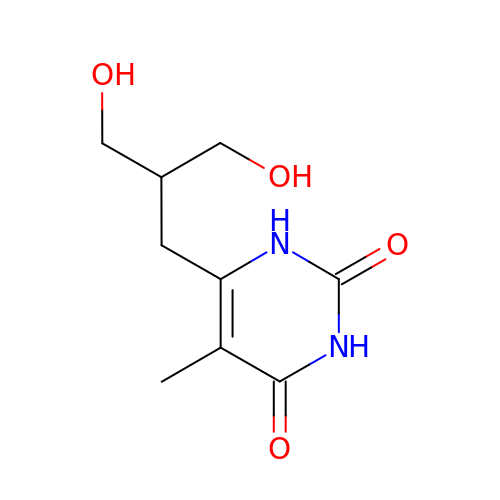6-[3-HYDROXY-2-(HYDROXYMETHYL)PROPYL]-5-METHYL-2,4(1H,3H)-PYRIMIDINEDIONE | C9 H14 N2 O4 | CLCPDSJUXHDRGX-UHFFFAOYSA-N> MAEQATKSVLFVCRGNKCRSPIAEAVFRKLVTDQNISENWVIDSGAVSDWNVGRSPDPRAVSCLRNHGIHTAHKARQITKEDFATFDYILCMDESNLRDLNRKSNQVKTCKAKIELLGSYDPQKQLIIEDPYYGNDSDFETVYQQCVRCCRAFLEKAH

LMW-PTP is a well-characterised phospho-tyrosine specific PTP, widely expressed in human tissues and conserved through evolution. The ligand-binding interface of LMW-PTP comprises the active site P-loop, the adjacent DPYY-loop (D-loop) and the variable region or variable loop. The catalytic residues C12 (nucleophile) and R18 (phosphate binding) are located in the P-loop, and D129 (general acid/base) in the D-loop. We demonstrate here that minimal re-design of LMW-PTP, by mutating only two residues, is sufficient to introduce new enzymatic activity towards four different phosphoinositide (PI) substrates.

Enzyme kinetics experiments for the dephosphorylation of phosphoinositides reveal that the RT, RTK and RKK mutant enzymes show selective specificity for PI5P, whereas RK has a broader specificity, with activity towards PI3P, PI4P, and PI5P and PI[3,5]P2, with the highest efficacy towards PI[3,5]P2. In order to assess the actual impact of the designed mutations on the protein structure, we determined the crystal structures of the I16K and L13R-I16K mutants at 1.8Å and 2.0Å resolution respectively. In both cases, the structures are similar to the WT enzyme with overall root-mean deviations (RMSDs) of 0.288 Å and 0.265 Å respectively. There are no structural distortions in main chain of the P-loop or the variable region, thus the mutations introduced do not alter the tertiary structure of the protein, consistent with a catalytically active enzyme. However, in both structures, the side chain of W49 is in the open position, away from the active site, thus confirming the flexibility of this side chain as suggested from the kinetics characterisation. In the structure of the RK mutant, the side chain of R13 points towards the centre of the active site interacting with a bound phosphate molecule and the catalytic D129. To evaluate if a PI molecule could fit in the crystal structure of the RK mutant, we performed docking with RosettaLigand using the PI[3,5]P2 ligand, and allowing the side chains of the protein residues in the binding interface (R13, I16, W49, N50, R53, Y131 and Y132) to be flexible. The ligand docks in the pocket, with the phosphorus atom of the D3 phosphate at a distance of 3.3Å from the sulphur atom of C12, similar to the 3.2Å distance observed in the MTMR2-PI[3,5]P2 complex. The new residues R13 and K16, both form interactions with the D5 and D1 phosphates respectively, and together with interactions with R53 they contribute to PI[3,5]P2 binding. The crystals structure of R13-K16 design shows a larger active site pocket than the WT enzyme, which is compatible with binding of PI substrates.> GIDPFTREDRIGVCKGIFRTDNVADDD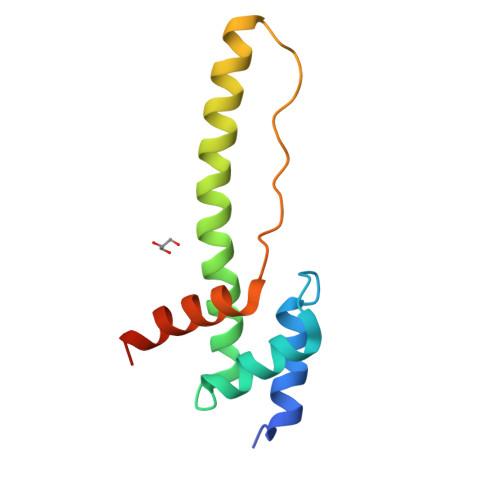IVKLVDTFPGQSIDFFGALRARVYDDEVRKWVSEVGVDTIGKKLVNSKEGPPSFEQPKMTIDKLLGYGGMLVQEQENVKR>[4x]MLGLLRRLFDNNEREIARYYKQVVEPVNRLEAEVEKLPDLAAAYRELKEKHEKGASLDELLPMAFALTRESAKRYLGMRHFDVQLIGGAVLHEGKIAEMKTGEGKTLVATLAVALNALTGKGVHVVTVNDYLARRDAEWMGPVYRGLGLSVGVIQHASTPAERRKAYLADVTYVTNSELGFDYLRDNMAISPDQLVLRHDHPLHYAIIDEVDSILIDEARTPLIISGPAEKATDLYYKMAEIAKKLERGLPAEPGVRKEPTGDYTVEEKNRSVHLTLQGIAKAEKLLGIEGLFSPENMELAHMLIQAIRAKELYHRDRDYIVQDGQVIIVDEFTGRLMPGRRYGEGLHQAIEAKEGVRIERENQTLATITYQNFFRLYEKRAGMTGTAKTEEKEFQEIYGMDVVVVPTNRPVIRKDFPDVVYRTEKGKFYAVVEEIAEKYERGQPVLVGTISIEKSERLSQMLKEPRLYLPRLEMRLELFKKASQKQQGPEWER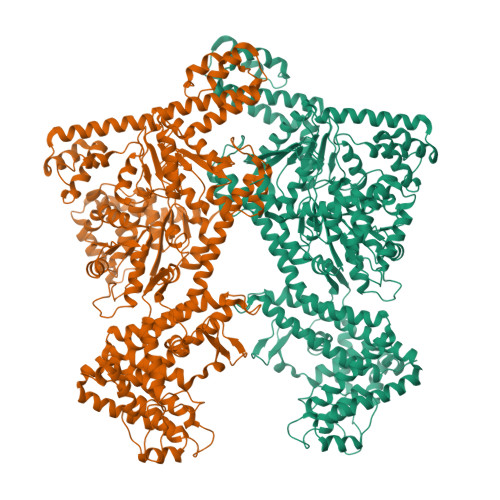LRKLLERPAQLKDEDLAPFEGLIPPKGNLRTAWEGLKRAVHTLAVLRQGIPHQVLNAKHHAREAEIVAQAGRSKTVTIATNMAGRGTDIKLGGNPEYLAAALLEKEGFDRYEWKVELFIKKMVAGKEEEARALAQELGIREELLERIREIREECKQDEERVRALGGLFIIGTERHESRRIDNQLRGRAGRQGDPGGSRFYVSFDDDLMRLFASDRVIAMLDRMGFDDSEPIEHPMVTRSIERAQKRVEDRNFAIRKQLLQFDDVLSRQREVIYAQRRLILLGKDEEVKEAAIGMVEETVASLAENFLNPEVHPEDWDLEGLKATLLDTAPQLQDFPFAELRALKAEEAVERLVEAALKAYEAREAELSPPLMRAVERFVILNVVDNAWKEHLHNLDVLRQGIFLRGYGQKDPFQEYKIEATRLFNEMVAFIKSEVAKFLFRLKVEAEPVRPVREAPYVPVPEAKPEPSEVFGVERKRATPPPQPGLSRAERRRLMRQEKKRKK> MGHHHHHHAMENKIEDIGQGAEIIKR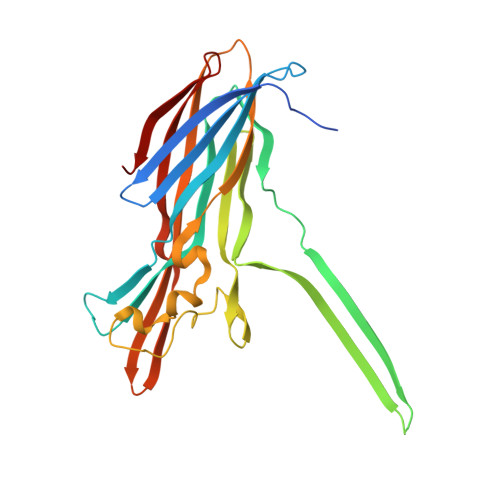TQDITSKRLAITQNIQFDFVKDKKYNKDALVVKMQGFISSRTTYSDLKKYPYIKRMIWPFQYNISLKTKDSNVDLINYLPKNKIDSADVSQKLGYNIGGNFQSAPSIGGSGSFNYSKTISYNQKNYVTEVESQNSKGVKWGVKANSFVTPNGQVSAYDQYLFAQDPTGPAARDYFVPDNQLPPLIQSGFNPSFITTLSHERGKGDKSEFEITYGRNMDATYAYVTRHRLAVDRKHDAFKNRNVTVKYEVNWKTHEVKIKSITPK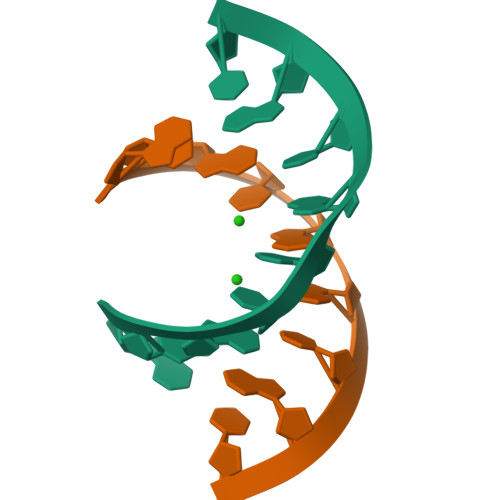>[12x]AUGUGGCAU> MVPTVQRGIIKMVLSGCAIIVRGQPRGGPPPERQINLSNIRAGNLARRAAATQPDAKDTPDEPWAFPAREFLRKKLIGKEVCFTIENKTPQGREYGMIYLGKDTNGENIAESLVAEGLATRREGMRANNPEQNRLSECEEQAKAAKKGMWSEGNGSHTIRDLKYTIENPRHFVDSHHQKPVNAIIEHVRDGSVVRALLLPDYYLVTV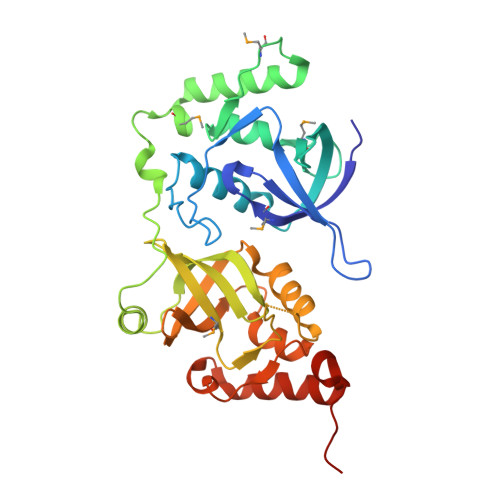MLSGIKCPTFRREADGSETPEPFAAEAKFFTESRLLQRDVQIILESCHNQNILGTILHPNGNITELLLKEGFARCVDWSIAVYTRGAEKLRAAERFAKERRLRIWRDYVAPTANLDQK> RAVDLVDDSNDVDNSIEAEEEKPRNRAFEADWLKFTKTPPTKLQQADGATIEIVCEMMGSQVPSIQWVVGHLPRSELDDLDSNQVAEEAPSAIVRVRSSHIIDHVLSEARTYTCVGRTGSKTIYASTVV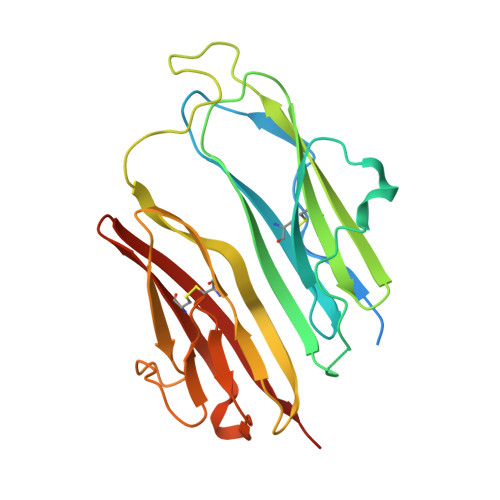HPPRSSRLTPEKTYPGAQKPRIIYTEKTHLDLMGSNIQLPCRVHARPRAEITWLNNENKEIVQGHRHRVLANGDLLISEIKWEDMGNYKCIARNVVGKDTADTFVYPVLNEED>GFVAKDDSLRTFFDAMALQLKEPVIVSKMAARKKITGNFEFHDPNALLEKLSLQLGLIWYFDGQAIYIYDASEMRNAVVSLRNVSLNEFNNFLKRSGLYNKNYPLRGDN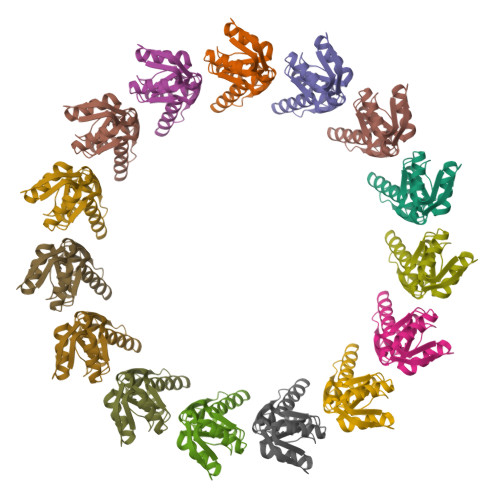RKGTFYVSGPPVYVDMVVNAATMMDKQN[15x]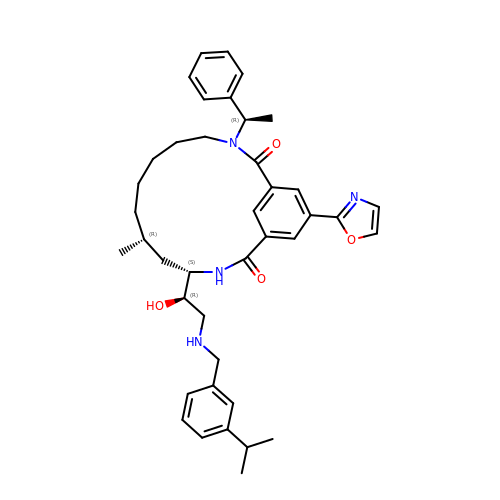(9R,11S)-11-[(1R)-1-hydroxy-2-({[3-(propan-2-yl)phenyl]methyl}amino)ethyl]-9-methyl-16-(1,3-oxazol-2-yl)-3-[(1R)-1-phenylethyl]-3,12-diazabicyclo[12.3.1]octadeca-1(18),14,16-triene-2,13-dione | C40 H50 N4 O4 | WTVYZBOJEASHJM-PMKGPLEQSA-N> SMTKPVGPWQDCAEARQAGHEQSGVYELRVGRHVVSVWCEQQLEGGGWTVIQRRQDGSVNFFTTWQHYKAGFGRPDGEYWLGLEPVYQLTSRGDHE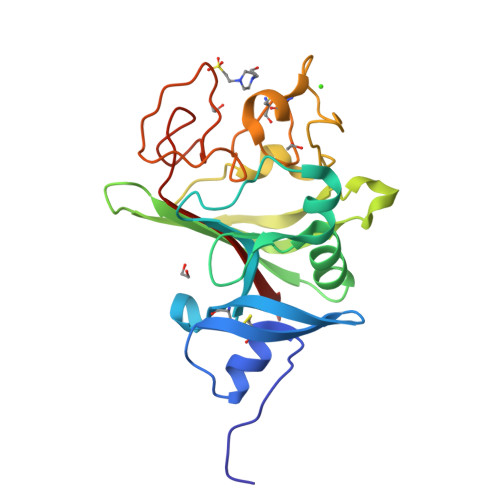LLVLLEDWGGRGARAHYDGFSLEPESDHYRLRLGQYHGDAGDSLSWHNDKPFSTVDRDRDSYSGNCALYQRGGWWYHACAHSNLNGVWHHGGHYRSRYQDGVYWAEFRGGAYSLRKAAMLIRPLKL> MRYGHFDDEAREYVITTPHTPYPWINYLGSEQFFSLLSHQAGGYSFYRDAKMRRLTRYRYNNIPADAGGRYLYVNDGGDVWTPSWLPVKADLDHFEARHGLGYSTITGERNGVRVETLFFVPVGENAEVQKVTVTNTSDSYKSLTLFSFVEFCLWNAQDDQTNYQRNLSIGEVEVEQESPHGSAIYHRTEYRERRDHYAVFAVNTQAEGFDTDRDTFVGAYNSLGEAAVPLKGESANSVASGWYPIGSHSVAVSLAPGESRELVYVLGYVENPDEEKWADDAKQVVNKERAHALLSRFATSEQTDAAFAALKDYWTDLLSTYSVSSNDEKLDRM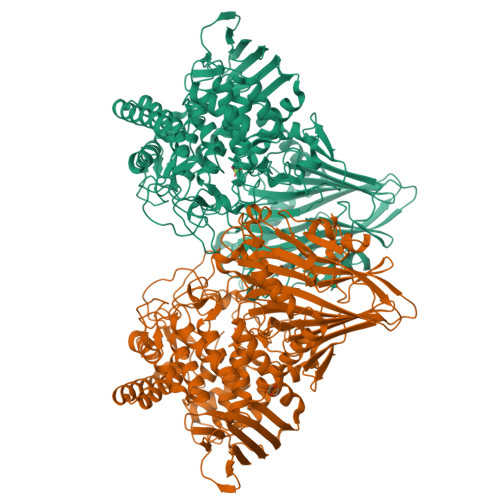VNIWNQYQCMVTFNMSRSASFFETGIGRGMGFRDSNQDLLGFVHLIPERARERIIDIASTQFADGSAYHQYQPLTKRGNNDIGSGFNDDPLWLIAGTAAYIKETGDFSILDEPVPFDNEPGSEVPLFEHLTRSFEFTVTHRGPHGLPLIGRADWNDCLNLNCFSTTPGESFQTIENQAGGVAESTFIAAQFVLYGEQYAELAARRGLADVADRARGHVAEMRDALLTDGWDGSWFLRAYDYYGNPIGTDAHDEGKIWIEPQGFAVMAGVGVGEGPQDTDAPAIKALDSVNEMLATDHGMVLQYPAYTTYQVHMGEVSTYPPGYKENGGIFCHANPWVIIAETVVGRGGRAFDYYKRITPAYREDISDVHRLEPYVYAQMIAGKEAVRHGEAKNSWLTGTAAWNFVTVSQYLLGVRPEYDGLVVDPQIGPDVPSFTVTRVARGATYEITVTNSGTDGSRGRLVVDGTPVEGNLVPYAPAGSTVRVDVTL> MRFKNVKKTALMLAMFGMATSSNAALFDYNATGDTEFDSPAKQGWMQDNTNNGSGVLTNADGMPAWLVQGIGGRAQWTYSLSTNQHAQASSFGWRMTTEMKVLSGGMITNYYANGTQRVLPIISLDSSGNLVVEFEGQTGRTVLATGTAATEYHKFELVFLPGSNPSASFYFDGKLIRDNIQPTASKQNMIVWGNGSSNTDGVAAYRDIKFEIQGDVIFRGPDRIPSIVASSVTPGVVTAFAEKRVGGGDPGALSNTNDIITRTSRDGGITWDTELNLTEQINVSDEFDFSDPRPIYDPSSNTVLVSYARWPTDAAQNGDRIKPWMPNGIFYSVYDVASGNWQAPIDVTDQVKERSFQIAGWGGSELYRRNTSLNSQQDWQSNAKIRIVDGAANQIQVADGSRKYVVTLSIDESGGLVANLNGVSAPIILQSEHAKVHSFHDYELQYSALNHTTTLFVDGQQITTWAGEVSQENNIQFGNADAQIDGRLHVQKIVLTQQGHNLVEFDAFYLAQQTPEVEKDLEKLGWTKIKTGNTMSLYGNASVNPGPGHGITLTRQQNISGSQNGRLIYPAIVLDRFFLNVMSIYSDDGGSNWQTGSTLPIPFRWKSSSILETLEPSEADMVELQNGDLLLTARLDFNQIVNGVNYSPRQQFLSKDGGITWSLLEANNANVFSNISTGTVDASITRFEQSD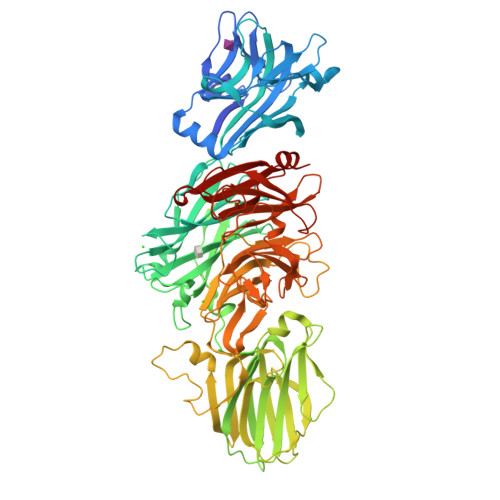GSHFLLFTNPQGNPAGTNGRQNLGLWFSFDEGVTWKGPIQLVNGASAYSDIYQLDSENAIVIVETDNSNMRILRMPITLLKQKLTLSQN> MDELGIPVYKRGFPEHLLRGYEFIIDVGTKIESVGGRHDVTKIPEMNAYDIKQESIRTALWYNPIRNDGFVLPRVLDITLRGYDERRAVVESTRHKSFHTNDQWVQWMMKDSMDAQPLKVGLDDQSRNVAHSLHNCVVKIDSKKADTMSYHVEPIEDASKGCLHTRTMMWNHLVRIETFHAAQEVAYTLKPTYDIVVHAERRDRSQPFRPGDQTLINFGRGQKVTMNHNSYDKMVEGLAHLVIRGKIPEVIRDDIASLDEICNRWIQSRHDPGEIKAYELCKILSTIGRKVLDREKEPEDEASLSIRFQEAIDNKFRQHDPERLKIFEHRNQRRDEDRFYILLMIAASDTFNTRVWWSNPYPCLRGTLIASETKLGDVYSMMRSWYDWSVRPTYTPYEKTREQEKYIYGRVN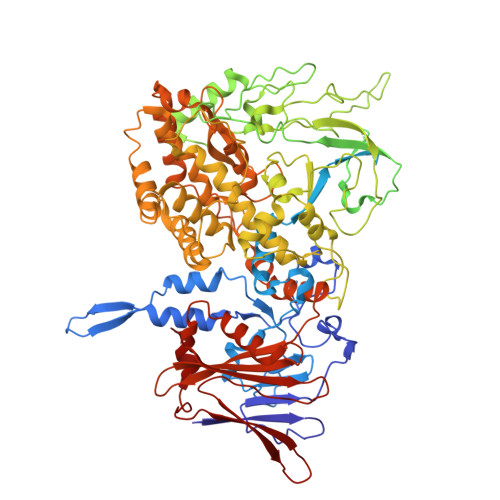LFDFVAEPGIKIVHWEYRLNHSTREITYAQGNPCDLYPEDDDVIVTKFDDVAYGQMINEMINGGWNQEQFKMHKILKSEGNVLTIDFEKDAKLTTNEGVTMPEYFNKWIIAPMFNAKLRIKHEEIAQRQSDDPMVKRTLSPITADPIELQRLTLARFYDIRPALRGQALSRQQAQSTYDEEISKRQDYAEILKRRGIVQIPKKPCPTVTAQYTLERYALFIISILQQHVVRDCDEEAVYEHPKADHELEIFGESIVDISQVIILAFDLIFERRRRVRDVYESRHIIARIRRMRGKERLNVIAEFFPTYGGLLNGLNSATVVQNIMYLNFLPLYFLVGDNMIYSHRQWSIPLLLYTHEVMVVPLEVGSYNDRCGLIAYLEYMVFFPSKAIRFSKLNEAQPKIAREMLKYYANTTVYDGGVNYNVVTTKQLLYETYLASLCGGISDGIVWYLPITHPNKCIVAIEVSDERVPASIRAGRIRLRFPLSARHLKGVVIIQIDEEGEFTVYSEGIVSHRVCKKNLLKYMCDIILLKFSGHVFGNDEMLTKLLNV> VESEFPYLLSLLG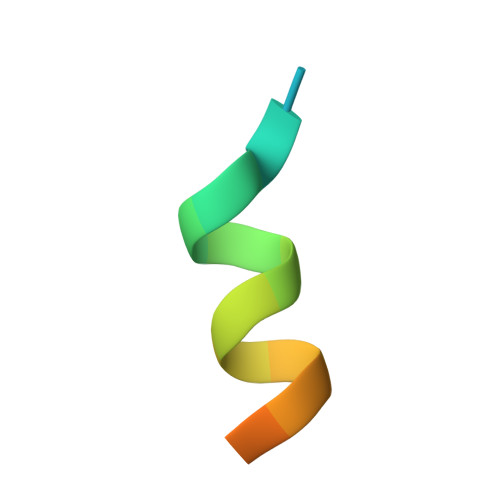EVSPQP> NDKICAGVASGKGTHRVETITKGEVLVTNAINMTHTPTSGPFGDLKTGNVRDKLCPTCTGCTDMDVALMTPTCNGVIPEAIAAIQHENRPLQSKCNPILHDLGNTRQLPNLLRKYKKIRKSSGIAFPLASYADQPVISNPSGNCRDGNGVESEFGSLLWLTGNTKGAITGETITITHQCNNDEVMVLVWGAWADLSATMNTIYGVTTPQTYVSNFPSGRFSMSPFLGN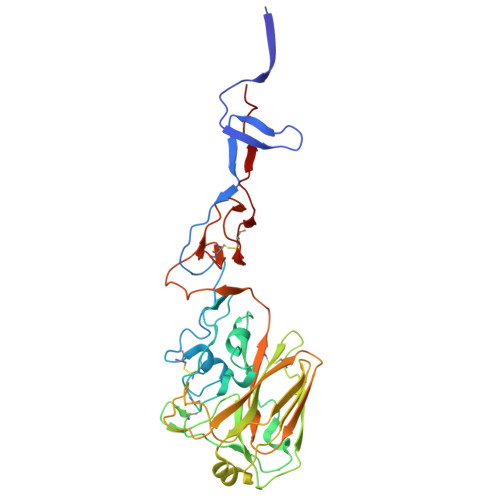FPALAETEATTATGRIYLRMEVLESGQRGTIQYQRGFMGPGKFWCLSEPIPVVKGAVKTNGAVSDCLHEVYGGISKPTPFYTGNRGKSVGNCPKWVRKPLLVVNGTKAR> SLNTGEPAPVLSSPPPADVSTFLAFPSPEKLLRLGPKSSVLIAQQTDTSDPEKVVSAFLKVSSVFKDEATVRMAVQDAVDALMQKAFNSSSFNSNTFLTRLLVHMGLLKSEDKVKAIANLYGPLMALNHMVQQDYFPKALAPLLLAFVTKPNSALESCSFARHSLLQTLYK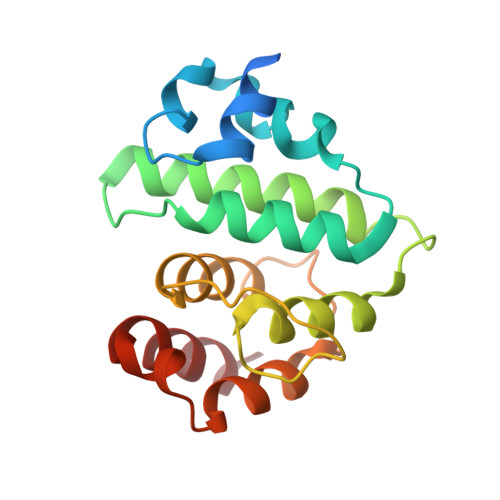V> MHHHHHHPEIVDTCSLASPASVCRTKHLHLRCSVDFTRRTLTGTAALTVQSQEDNLRSLVLDTKDLTIEKVVINGQEVKYALGERQSYKGSPMEISLPIALSKNQEIVIEISFETSPKSSALQWLTPEQTSGKEHPYLFSQCQAIHCRAILPCQ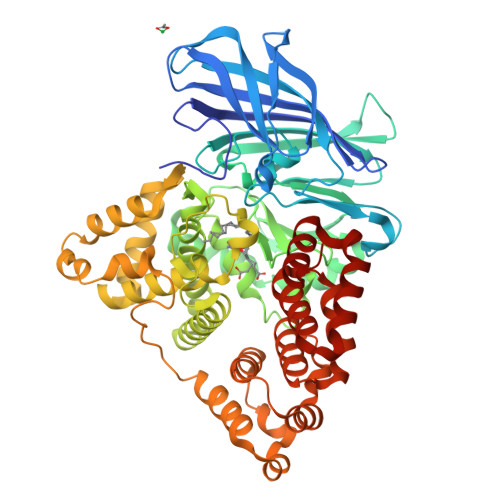DTPSVKLTYTAEVSVPKELVALMSAIRDGETPDPEDPSRKIYKFIQKVPIPCYLIALVVGALESRQIGPRTLVWSEKEQVEKSAYEFSETESMLKIAEDLGGPYVWGQYDLLVLPPSFPYGGMENPCLTFVTPTLLAGDKSLSNVIAHEISHSWTGNLVTNKTWDHFWLNEGHTVYLERHICGRLFGEKFRHFNALGGWGELQNSVKTFGETHPFTKLVVDLTDIDPNVAYSSVPYEKGFALLFYLEQLLGGPEIFLGFLKAYVEKFSYKSITTDDWKDFLYSYFKDKVDVLNQVDWNAWLYSPGLPPIKPNYDMTLTNACIALSQRWITAKEDDLNSFNATDLKDLSSHQLNEFLAQTLQRAPLPLGHIKRMQEVYNFNAINNSEIRFRWLRLCIQSKWEDAIPLALKMATEQGRMKFTRPLFKDLAAFDKSHDQAVRTYQEHKASMHPVTAMLVGKDLKVD2H-1,4-benzothiazin-3-amine | C8 H8 N2 S | 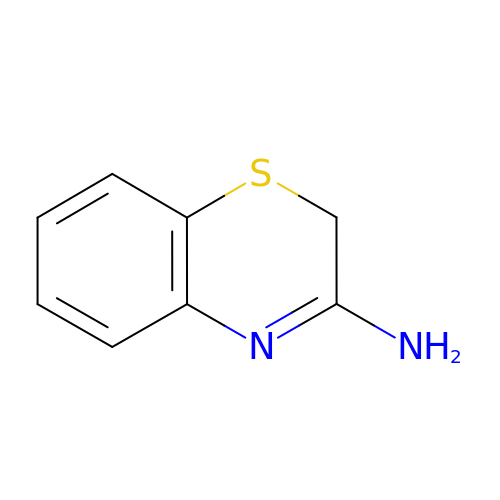SBZQHWWTOVFQFD-UHFFFAOYSA-N2-{[(4R)-2,5-dioxo-4-(4-pyridin-3-ylphenyl)imidazolidin-4-yl]methyl}-6-methoxy-1-oxo-1H-isoindolium 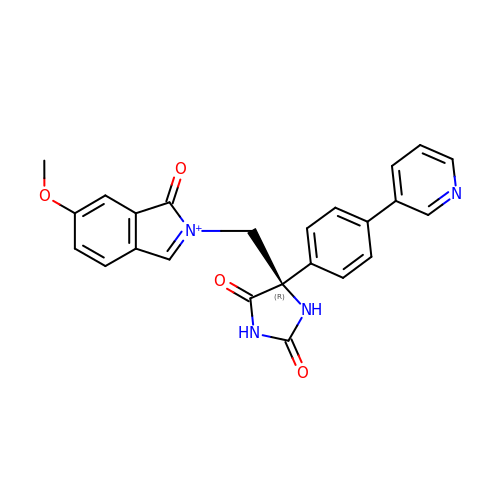| C24 H19 N4 O4 | IPWWTFLYEBQOPS-DEOSSOPVSA-O> GSVGNREEKILNREIGFAIGMPVCEFDMVKDPEVQDFRRNILNVCKEAVDLRDLNSPHSRAMYVYPPNVESSPELPKHIYNKLDKGQIIVVIWVIVSPNNDKQKYTLKINHDCVPEQVIAEAIRKKTRSMLLSSEQLKLCVLEYQGKYILKVCGCDEYFLEKYPLSQYKYIRSCIMLGRMPNLMLMAKESLYSQLPMDCFTMPSYSRRISTATPYMNGETSTKSLWVINSALRIKILCATYVNVNIRDIDKIYVRTGIYHGGEPLCDNVN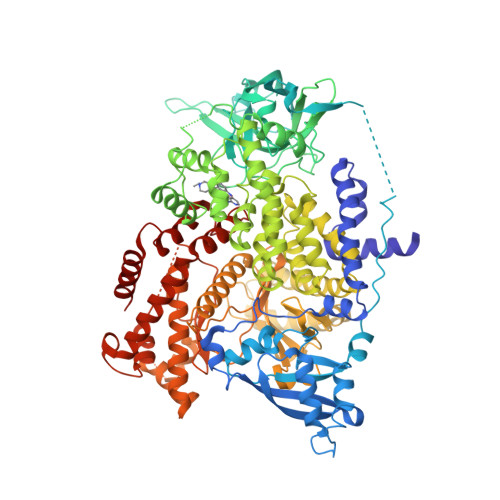TQRVPCSNPRWNEWLNYDIYIPDLPRAARLCLSICSVKGRKGAKEEHCPLAWGNINLFDYTDTLVSGKMALNLWPVPHGLEDLLNPIGVTGSNPNKDTPCLELEFDWFSSVVKFPDMSVIEEHANWSVSREAGFSYSHAGLSNRLARDNELRENDKEQLKAISTRDPLSEITEQEKDFLWSHRHYCVTIPEILPKLLLSVKWNSRDEVAQMYCLVKDWPPIKPEQAMELLDCNYPDPMVRGFAVRCLEKYLTDDKLSQYLIQLVQVLKYEQYLDNLLVRFLLKKALTNQRIGHFFFWHLKSEMHNKTVSQRFGLLLESYCRACGMYLKHLNRQVEAMEKLINLTDILKQEKKDETQKVQMKFLVEQMRRPDFMDALQGFLSPLNPAHQLGNLRLEECRIMSSAKRPLWLNWENPDIMSELLFQNNEIIFKNGDDLRQDMLTLQIIRIMENIWQNQGLDLRMLPYGCLSIGDCVGLIEVVRNSHTIMQIQCKGGLKGALQFNSHTLHQWLKDKNKGEIYDAAIDLFTRSCAGYCVATFILGIGDRHNSNIMVKDDGQLFHIDFGHFLDHKKKKFGYKRERVPFVLTQDFLIVISKGAQECTKTREFERFQEMCYKAYLAIRQHANLFINLFSMMLGSGMPELQSFDDIAYIRKTLALDKTEQEALEYFMKQMNDAHH>[6x]MENKFDHMKLENQLSFLLYASSRE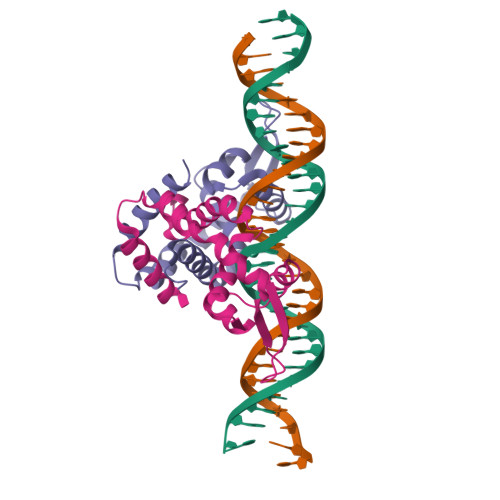MTKQYKPLLDKLNITYPQYLALLLLWEHETLTVKKMGEQLYLDSGTLTPMLKRMEQQGLITRKRSEEDERSVLISLTEDGALLKEKAVDIPGTILGLSKQSGEDLKQLKSALYTLLETLHQKN> MTKQLPNLQVALDHSNLKGAITAAVSVGNEVDVIEAGTVCLLQVGSELVEVLRSLFPDKIIVADTKCADAGGTVAKNNAVRGADWMTC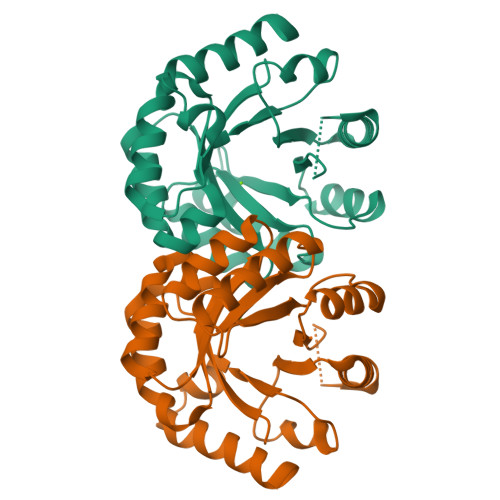ICSATIPTMKAARKAIEDINPDKGEIQVELYGDWTYDQAQQWLDAGISQAIYHQSRDALLAGETWGEKDLNKVKKLIEMGFRVSVTGGLSVDTLKLFEGVDVFTFIAGRGITEAKNPAGAARAFKDEIKRIWG O-methyl-N-[(2S)-4-methyl-2-(sulfanylmethyl)pentanoyl]-L-tyrosine | C17 H25 N O4 S 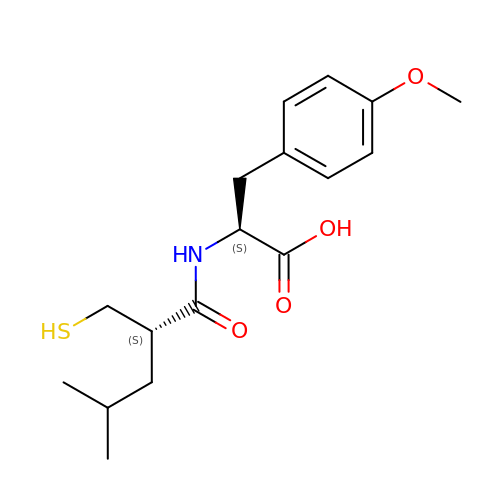| PRPWYZNFKBFGFI-HIFRSBDPSA-N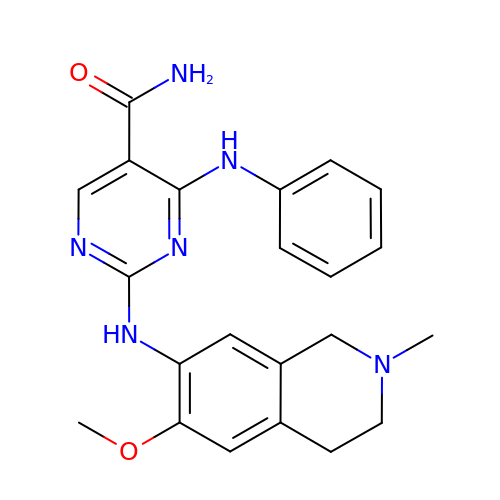4-anilino-2-[(6-methoxy-2-methyl-1,2,3,4-tetrahydroisoquinolin-7-yl)amino]pyrimidine-5-carboxamide | C22 H24 N6 O2 | GECWYEGIHOUDQU-UHFFFAOYSA-N> GHMASGLTIYFKKPDSWGTPHLYYYDTNPKVDEPTWSEAPEMEHYEGDWYTHTIEGVESV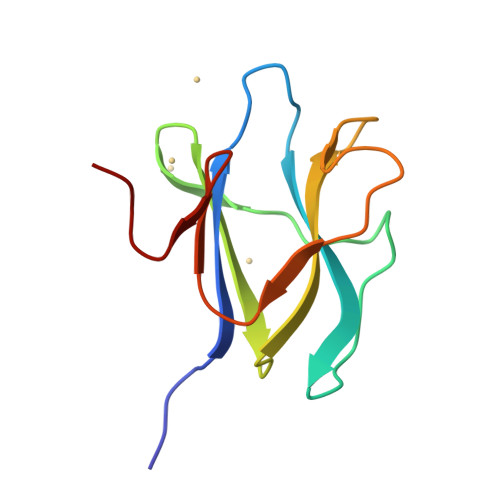RLLFKDRGTNQWPGPGEPGFFRDQDGWFDGEWHVDRPG>HHHHHHMKTTPGPVMLDVVGTTLSRDDARRLAHPNTGGVILFARHFQNRAQLTALTDSIRAVREDILIAVDHEGGRVQRFRTDGFTVLPAMRRLGELWDRDVLLATKVATAVGYILAAELRACGIDMSFTPVLDLDYGHSKVIGDRAFHRDPRVVTLLAKSLNHGLSLAGMANCGKHFPGHGFAEADSHVALPTDDRTLDAILEQDVAPYDWLGLSLAAVIPAHVIYTQVDKRPAGFSRVWLQDILRGKLGFTGAIFSDDLSMEAAREGGTLTQAADAA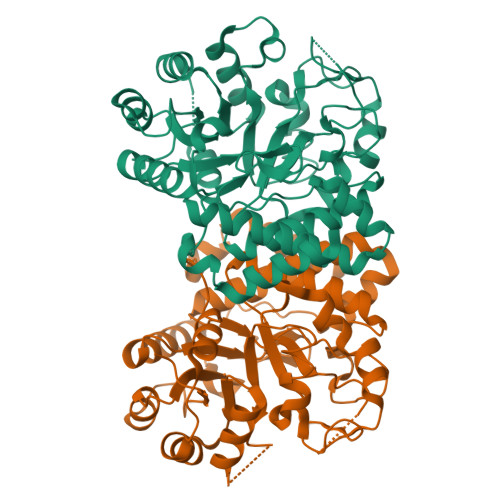LAAGCDMVLVCNQPDAAEVVLNGLKARASAESVRRIKRMRARGKALKWDKLIAQPEYLQAQALLSSALA[2x]> MSKVMKPSNGKGSRKSSKAATPDTKNFFHAKKKDPVNQDKANNASQITPTVPHSHPSDMVIPDHLAELIPELYSFQQLVDSEKRLDHFIHLRNLHMKRMVAQWERSKLSQEFLYPHLNFPNVKFLRIFISNVSENQPWQMDTNNEADLMALENATWTMRIEGRLLDNVQANDPAREKFSSFIESIVVDFKNKENDNVPSTKFNAAPEENATEGPSDKKLNLNLPLQFSLPNGDNSTTTNTDQNNATMGEETAKKDMSSTTPKLESVKWQYDPNNPVDFDGLDIKRVGSENVECTISILRKSSPEEPFMSYSPQLTAIIGLKSGTSHDAIFSIYKYIHLNELLTNDESAFENLMGNRNNHNSNTSTSKMLDAASSQVSIVKLDTQLITLLPSSLKESSPDTMKLTDLLSLINSTHLLPLQPIEIDYTVRVDKASTYGELVLDIEVPDVNALKFNNTQRESQIGAAELNENARELEQIKPKIALQDKEITSVLSNLHESNKRYRFFKKISEDPVKALN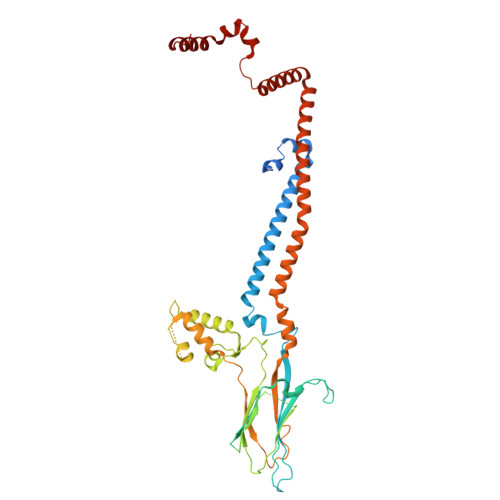ECIASTSNALKVLSGDEGYNEDMVRRANFYKENEAMLRENIEVILSNGRM> VPQKPKVSLNPPWNRIFK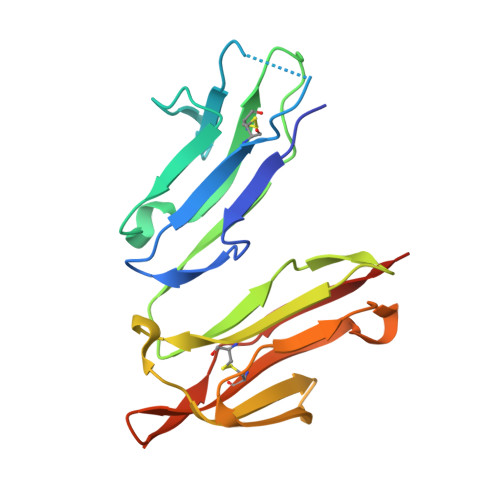GENVTLTCNGNNFFEVSSTKWFHNGSLSEETNSSLNIVNAKFEDSGEYKCQHQQVNESEPVYLEVFSDWLLLQASAEVVMEGQPLFLRCHGWRNWDVYKVIYYKDGEALKYWYENHNISITNATVEDSGTYYCTGKVWQLDYESEPLNITVIKAPREK>GAMASELTPEERSELKNSIAEFHTYQLDPGSCSSLHAQRIHAPPELVWSIVRRFDKPQTYKHFIKSCSVEQNFEMRVGCTRDVIVISGLPANTSTERLD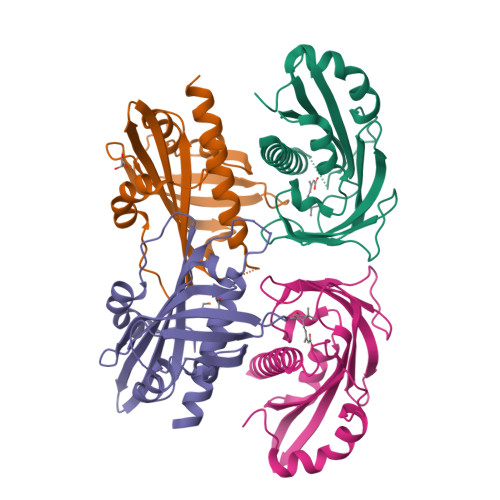ILDDERRVTGFSIIGGEHRLTNYKSVTTVHRFEKENRIWTVVLESYVVDMPEGNSEDDTRMFADTVVKLNLQKLATVAEAMARNSGDGSGSQVT[4x]>ADPKCTVSHEVADCSHLKLTQVPDDLPTNITVLNLTHNQLRRLPAANFTRYSQLTSLDVGFNTISKLEPELCQKLPMLKVLNLQHNELSQLSDKTFAFCTNLTELHLMSNSIQKIKNNPFVKQKNLITLDLSHNGLSSTKLGTQVQLENLQELLLSNNKIQALKSEELDIFANSSLKKLELSSNQIKEFSPGCFHAIGRLFGLFLNNVQLGPSLTEKLCLELANTSIRNLSLSNSQLSTTSNTTFLGLKWTNLTMLDLSYNNLNVVGNDSFAWLPQLEYFFLEYNNIQHLFSHSLHGLFNVRYLNLKRSFTKQSISLASLPKIDDFSFQWLKCLEHLNMEDNDIPGIKSNMFTGLINLKYLSLSNSFTSLRTLTNETFVSLAHSPLHILNLTKNKISKIESDAFSWLGHLEVLDLGLNEIGQELTGQEWRGLENIFEIYLSYNKYLQLTRNSFALVPSLQRLMLRRVALKNVDSSPSPFQPLRNLTILDLSNNNIANINDDMLEGLEKLEILDLQHNNLARLWKHANPGGPIYFLKGLSHLHILNLESNGFDEIPVEVFKDLFELKIIDLGLNNLNTLPASVFNNQVSLKSLNLQKNLITSVEKKVFGPAFRNLTELDMRFNPFDCTCESIAWFVNWINETHTNIPELSSHYLCNTPPHYHGFPVRLFDTSS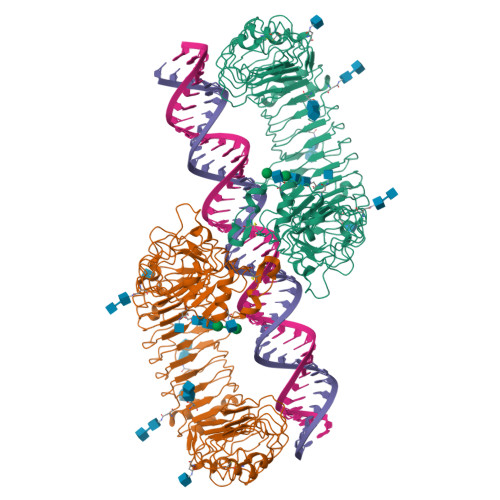CKSGRLVPRGSHHHHHH[2x]> MAITLFLD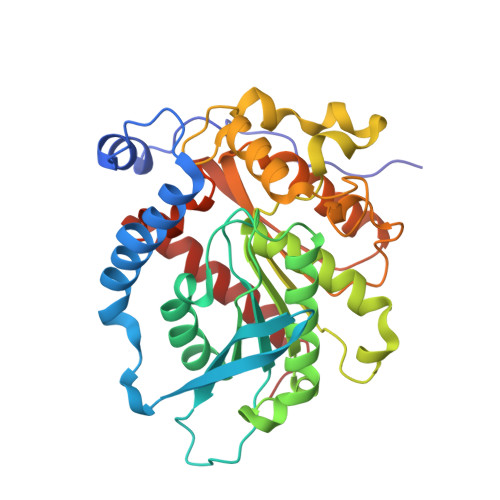EGLSTAHPEFAPVWAAFPQPTDPFPPLEARRAFWDEVVIPNLNKFLEPSLPSEDRYRLEDYYIPVEGTNMHVRTYIPTSSPDKTKTYPLLYWVHCGGWAIGNYEMDDYDLRIICDKLQVCAVSIDYRLTPESSSPTGAKDVYAGLKWAAANAGSFNADPKKGFVIAGQSAGGNLSLIAAHWARDDPFFANTPLTGQLVQYPPTCHPEAMPEEYKSCIKSMEECRDAPLLSKKEVYWFNELANPADPHDPSFSPLLFPSHANLPPLFFMSCGWDPLRDEGLLYHALVKEAGVETRMTMYPGVPHAFHMLFRSMKLAQKFQEETIEGMSWLFSKTPQ> AIPWGGNLEEVLEELEMALLAADVGLSATEEILQEVRASGRKDLKEAVKEKLVGMLEPDERRATLRKLGFNPQKPKPVEPKGRVVLVVGVNGVGKTTTIAKLGRYYQNLGKKVMFCAGDTFRAAGGTQLSEWGKRLSIPVIQGPEGTDPAALAYDAVQAMKARGYDLLFVDTAGRLHTKHNLMEELKKVKRAIAKADPEEPKEVWLVLDAVTGQNGLEQAKKFHEAVGLTGVIVTKLDGTAKGGVLIPIVRTLKVPIKFVGVGEG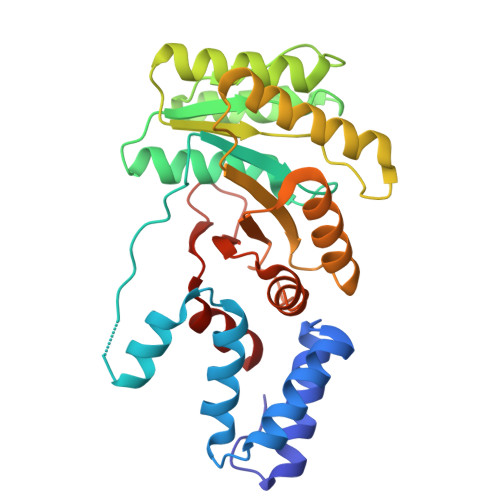PDDLQPFDPEAFVEALLED>[12x]MSKTESYCLEDALNDLFIPETTIETILKRLTIKKNIILQGPPGVGKTFVARRLAYLLTGEKAPQRVNMVQFHQSYSYEDFIQGYRPNGVGFRRKDGIFYNFCQQAKEQPEKKYIFIIDEINRANLSKVFGEVMMLMEHDKRGENWSVPLTYSENDEERFYVPENVYIIGLMNTADRSLAVVDYALRRRFSFIDIEPGFDTPQFRNFLLNKKAEPSFVESLCQKMNELNQEISKEATILGKGFRIGHSYFCCGLEDGTSPDTQWLNEIVMTDIAPLLEEYFFDDPYKQQKWTNKLLGDSSGSHHHHHH;>MEQPVIPVRNIYYMLTYAWGYLQEIKQANLEAIPGNNLLDILGYVLNKGVLQLSRRGLELDYNPNTEIIPGIKGRIEFAKTIRGFHLNHGKTVSTFDMLNEDTLANRIIKSTLAILIKHEKLNSTIRDEARSLYRKLPGISTLHLTPQHFSYLNGGKNTRYYKFVISVCKFIVNNSIPGQNKGHYRFYDFERNEKEMSLLYQKFLYEFCRRELTSANTTRSYLKWDASSISDQSLNLLPRMETDITIRSSEKILIVDAKYYKSIFSRRMGTEKFHSQNLYQLMNYLWSLKPENGENIGGLLIYPHVDTAVKHRYKINGFDIGLCTVNLGQEWPCIHQELLDIFDEYLK[2x]

McrBC is an antiphage defense system of Escherichia coli that specifically cleaves invading DNA that are methylated. Furthermore, upon binding of the endonuclease McrC, a higher oligomeric form—tetradecamers of 12 McrB and 2 McrC protomers—is formed. GTP hydrolysis by McrBC bound to a recognition sequence powers DNA translocation, and convergence of two such complexes on the DNA results in nucleolytic cleavage. Here we present the structure of the AAA+ domain of McrB in complex with McrC at 3.6 Å resolution using cryo-electron microscopy (cryo-EM), which reveals the coupling between the endonuclease and the motor and the mechanism of activation of the GTPase.

The complex was formed in the presence of the GTP analog 5’-guanylyl imidodiphosphate (GNP). McrBΔNC is dumbbell shaped with the two hexameric McrBΔN rings tilted with respect to each other and sandwiching an McrC dimer. Three-dimensional (3D) classification resulted in nine major classes with varying tilt angle, indicative of conformational plasticity. The two protomers of McrC in the McrBΔNC complex are related to each other by a two-fold symmetry. The dimeric interface mainly constitutes helix H9 and has a total buried surface area of ~3000 Å2. The catalytic residues, Asp244, Asp257, and Lys259, are located close to the dimeric interface and aligned along the FA interface of McrB. A particularly interesting feature of McrBΔNC is that the McrC stalk blocks the pore of the McrB ring.> MVPISPIETVPVKLKPGMDGPKVKQWPLTEEKIKALVEICTEMEKEGKISKIGPENPYNTPVFAIKKKDSTKWRKLVDFRELNKRTQDFWEVQLGIPHPAGLKKKKSVTVLDVGDAYFSVPLDEDFRKYTAFTIPSINNETPGIRYQYNVLPQGWKGSPAIFQSSMTKILEPFKKQNPDIVIYQYMDDLYVGSDLEIGQHRTKIEELRQHLLRWGLTTPDKKHQKEPPFLWMGYELHPDKWTVQPIVLPEKDSWTVNDIQKLVGKLNWASQIYPGIKVRQLSKLLRGTKALTEVIPLTEEAELELAENREILKEPVHGVYYDPSKDLIAEIQKQGQGQWTYQIYQEPFKNLKTGKYARMRGAHTNDVKQLTEAVQKITTESIVIWGKTPKFKLPIQKETWETWWTEYWQATWIPEWEFVNTPPLVKLWYQL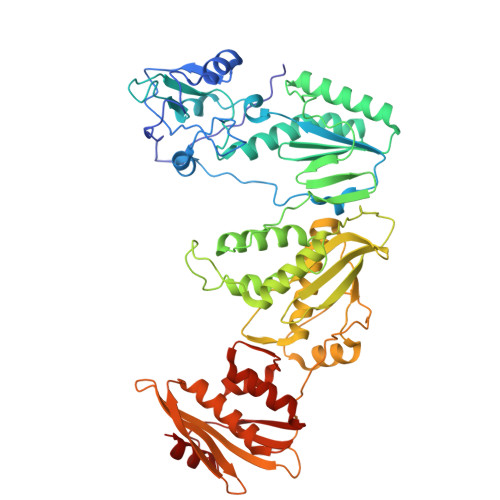EKEPIVGAETFYVDGAANRETKLGKAGYVTNKGRQKVVPLTNTTNQKTELQAIYLALQDSGLEVNIVTNSQYALGIIQAQPDKSESELVNQIIEQLIKKEKVYLAWVPAHKGIGGNEQVDKLVSA>[4x]GAMGARRRRKPRVLFSQAQVYELERRFKQQRYLSAPERDQLASVLKLTSTQVKIWFQNRRYKSKRQRQSSSSSSSSSSSSSSSAMEGIKVFLHERELWLKFHEVGTEMIITKAGRRMFPSYKVKVTGLNPKTKYILLMDIVPADDHRYKFADNKWSVTGKAEPAMPGRLYVHPDSPATGAHWMRQLVSFQKLKLTNNHLDPFGH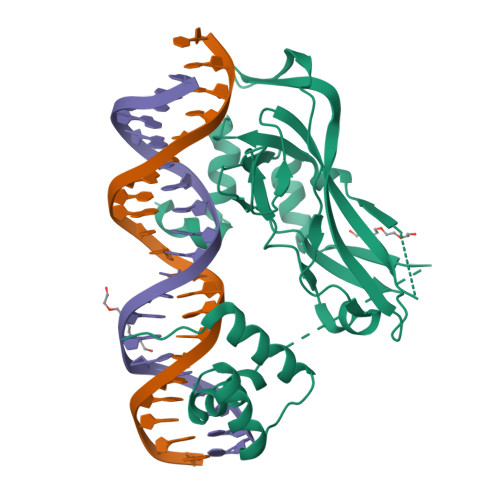IILNSMHKYQPRLHIVKADENNGFGSKNTAFSTHVFPETAFIAVTSYQNHKITQLKIENNPFAKGFRGSDDLELHRMSRMQ Two enzymes, peptidylglycine α-hydroxylating monooxygenase (PHM; EC 1.14.17.3) and peptidyl-α-hydroxyglycine α-amidating lyase (PAL; EC 4.3.2.5) working sequentially are the only proteins known to catalyze this reaction. PHM, a two Cu enzyme, catalyzes the stereospecific hydroxylation of the glycine Cα of peptidylglycine substrates. The two copper atoms in PHM, CuH, and CuM (located in the N- and C-subdomains, respectively), each use a single reducing equivalent from ascorbate to catalyze the reduction of molecular oxygen for the hydroxylation of the Cα of glycine at the carboxy-terminus of the peptide substrate. Crystallographic data on apo wild-type PHM and on several crystal forms of three CuH mutants (H107A, H108A, and H172A) presented here show that the copper ions are required not only for the catalytic steps but also for substrate binding and for locking the overall conformation of PHM in a configuration that is catalytically active.

The structure of the H107A mutant crystallized in the same conditions as the wild-type is highly similar to that of wild-type PHM. The structure, except for the lack of Cu2+ in the CuH site, is very similar to that of wild-type PHM (RMSD = 0.42 Å for 283 Cα carbons). Despite lacking its Cu2+, the rest of the CuH site shows little change except for the absence of the side chain of residue 107. The mutant does have Cu2+ in the CuM site and the geometry of the coordination is almost identical to that of wild-type PHM. The main difference is a small (<0.5 Å) narrowing of the space between the two domains. The coordination of the copper at the CuM site remains unchanged and even the two remaining histidines at CuH site show only minor changes.

> NECLGTIGPVTPLDASDFALDIRMPGVTPKESDTYFCMSMRLPVDEEAFVIDFKPRASMDTVAHMLLFGCNMPSSTGSYWFCDEGTCTDKANILYAWARNAPPTRLPKGVGFRVGGETGSKYFVLQVHYGDISAFRDNHKDCSGVSVHLTRVPQPLIAGMYLMMSVDTVIPPGEKVVNADISCQYKMYPMHVFAYRVHTHHLGKVVSGYRVRNGQWTLIGRQNPQLPQAFYPVEHPVDVTFGDILAARCVFTGEGRTEATHIGGTSSDEMCNLYIMYYMEAKYALSFMTCTKNVAPDMFRTIPAEANIPIPV(1E)-4-oxobut-1-ene-1,2,4-tricarboxylic acid | C7 H6 O7 | 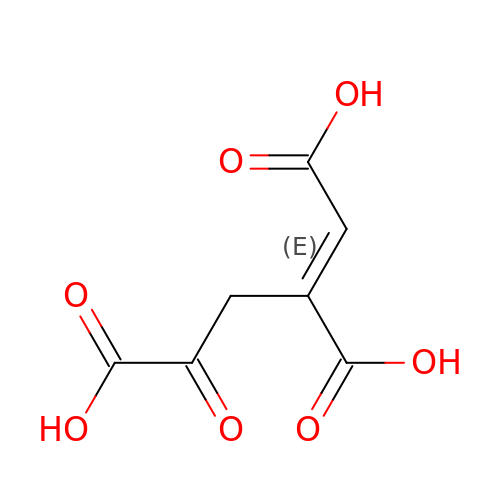ODTDYYZJDQGKQT-NSCUHMNNSA-N>[4x]GHMKASSRRTISQNKRRYRKDGFDLDLTYVTDHVIAMSFPSSGRQSLFRNPIGEVSRFFKTKHPDKFRIYNLCSERGYDETKFDNHVYRVMIDDHNVPTLVDLLKFIDDA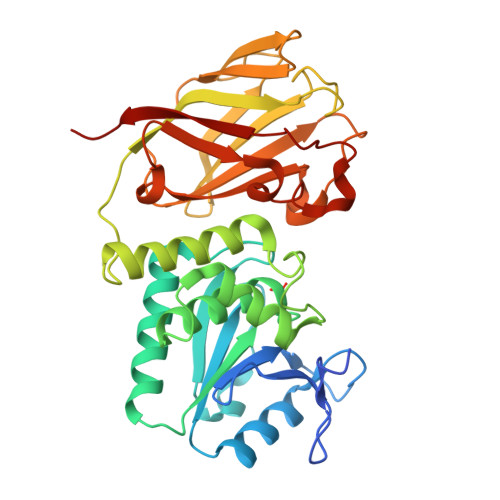KVWMTSDPDHVIAIHSKGGKGRTGTLVSSWLLEDGKFDTAKEALEYFGSRRTDFEVGDVFQGVETASQIRYVGYFEKIKKNYGGQLPPMKKLKVTGVTITAIQGVGRGNGSDLSMQIVSERQEVLLCKFAEGYNCALQYDATDDCVTCEVKNCPVLAGDIKVRFMSTSKSLPRGYDNCPFYFWFNTSLVEGDHVTLKREEIDNPHKKKTWKIYRDNFTVKLTFSDAEDI> GTTVS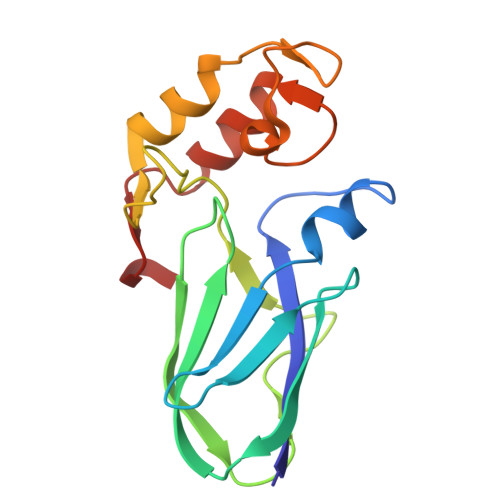GYINPDFVTTSTTAPIVKAGFTVEIVGTTKSAVTDSNGYFEIKDVAAGTYTVKITKANYLTREIANVSVTADKELSTSASPILMWAGDMAIGGTQDGAINLEDILEICKAFNTSSTDAKYQVGLDLNRDGAISLEDVMIVAKHFGKVSSDY>[8x]MSLKITRIDIHRTDLPVRGGVYRLSGGREYHSYDATIVSIETDTGLTGWGESTPFGSTYIAAHAGGTRAALELLAPAILGMDPRQHDRIWDRMRDTLKGHRDARAALDIACWDIAAQAAGLPLCDMTGGRVAGPVPVISSIGGDTPE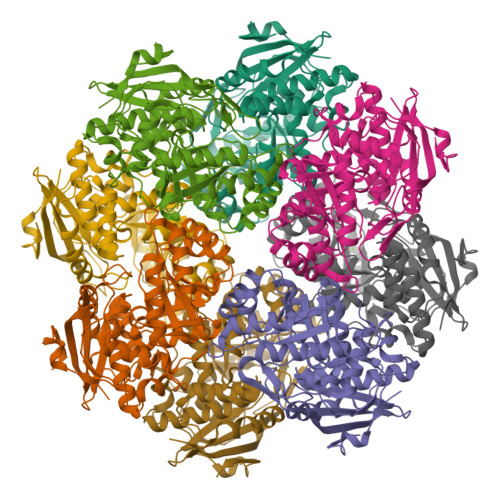AMRAKVARHRAQGFKGHSIKIGASEAEGGPALDAERITACLADRQPGEWYLADANNGLTVEHALRMLSLLPPGLDIVLEAPCASWAETKSLRARCALPLLLDELIQTETDLIAAIRDDLCDGVGLKVSKQGGITPMLRQRAIAAAAGMVMSVQDTVGSQISFAAILHLAQSTPRHLLRCALDTRAMTTAELAEIDAPLRDGGASAPSDPGLGLRVNRDALGTPVKTFGDPIEGHHHHHH3-[2-(4-fluoranylphenoxy)ethyl]-1,3-diazaspiro[4.5]decane-2,4-dione | C16 H19 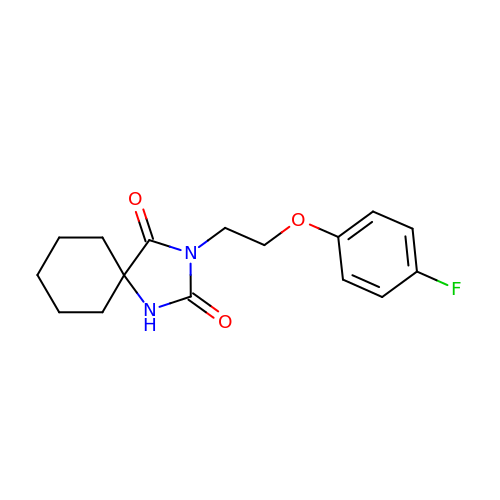F N2 O3 | WWRSQXLLQVERHE-UHFFFAOYSA-N> IVCHTTATSPISAVTCP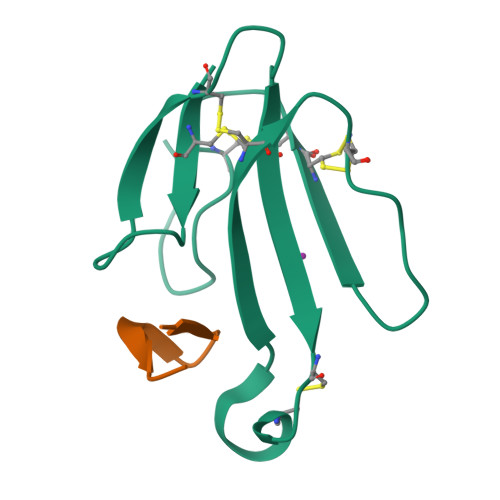PGENLCYRKMWCDVFCSSRGKVVELGCAATCPSKKPYEEVTCCSTDKCNPHPKQRPG;> IVCHTTATSPISAVTCPPGENLCYRKMWCDAFCSSRGKVVELGCAATCPSKKPYEEVTCCSTDKCNPHPKQRPG;>[2x]WRYYESSLLPYPD> YGPPGPPGPPGPPGLKGHNGLPGPPG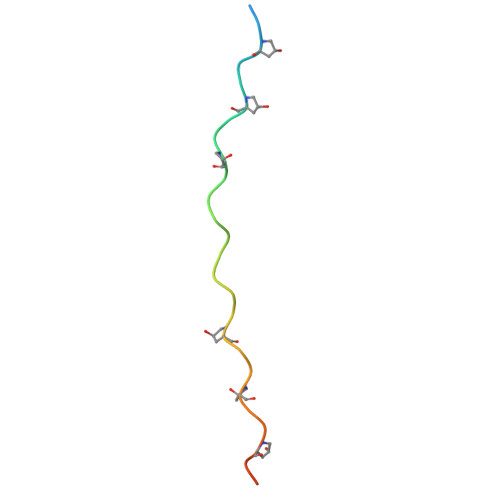PPGPPGPCG>[2x]MSEFNITETYLRFLEEDTEMTMPIAAIEALVTLLRIKTPETAAEMINTIKSSTEELIKSIPNSVSLRAGCDIFMRFVLRNLHLYGDWENCKQHLIENGQLFVSRAKKSRNKIAEIGVDFIADDDIILVHGYSRAVFSLLNHAANKFIRFRCVVTESRPSKQGNQLYTLLEQKGIPVTLIVDSAVGAVIDKVDKVFVGAEGVAESGGIINLVGTYSVGVLAHNARKPFYVVTESHKFVRMFPLSSDDLPMAGPPLDFTRRTDDLEDALRGPTIDYTAQEYITALITDLGVLTPSAVSEELIKMWYD;>[2x]MSSQAFTSVHPNAATSDVNVTIDTFVAKLKRRQVQGSYAIALETLQLLMRFISAARWNHVNDLIEQIRDLGNSLEKAHPTAFSCGNVIRRILAVLRDEVEEDTMSTTVTSTSVAEPLISSMFNLLQKPEQPHQNRKNSSGSSSMKTKTDYRQVAIQGIKDLIDEIKNIDEGIQQIAIDLIHDHEILLTPTPDSKTVLKFLITARERSNRTFTVLVTEGFPNNTKNAHEFAKKLAQHNIETLVVPDSAVFALMSRVGKVIIGTKAVFVNGGTISSNSGVSSVCECAREFRTPVFAVAGLYKLSPLYPFDVEKFVEFGGSQRILPRMDPRKRLDTVNQITDYVPPENIDIYITNVGGFNPSFIYRIAWDNYKQIDVHLDKNKA;>[2x]MSIQAFVFCGKGSNLAPFTQPDFPFQTQNKDSTAATSGDKLNELVNSALDSTVINEFMQHSTRLPKALLPIGNRPMIEYVLDWCDQADFKEISVVAPVDEIELIESGLTSFLSLRKQQFELIYKALSNSNHSHHLQDPKKINFIPSKANSTGESLQKELLPRINGDFVILPCDFVTDIPPQVLVDQFRNRDDNNLAMTIYYKNSLDSSIDKKQQQKQKQQQFFTVYSENEDSERQPILLDVYSQRDVTKTKYLQIRSHLLWNYPNLTVSTKLLNSFIYFCSFELCQLLKLGPQSMSRQASFKDPFTGNQQQQNPPTTDDDEDRNHDDDDDYKPSATSIQPTYFKKKNDLILDPINCNKSLSKVFRDLSRRSWQHSKPREPIGIFILPNETLFIRANNLNAYMDANRFVLKIKSQTMFTKNIQIQSAAIGADAIVDPKCQISAHSNVKMSVLGTQANIGSRCRVAGSLLFPGVHLGDEVILENCIIGPMAKIGSKCKLSNCYIEGHYVVEPKNNFKGETLANVYLDEDEEDELIYDDSVIAGESEIAEETDSDDRSDEDSDDSEYTDEYEYEDDGLFER;>MSESEAKSRSATPPSKAKQATPTTTAAANGEKKLTNKELKELKKQEKAAKRAAMKQANGISIEQQQQQAQMKKEKKQLQREQQQKREQKQKNANKKKQNERNVKKSTLFGHLETTEERRATILALTSAVSSPKTSRITAAGLMVPVVASALSGSNVLTASSLMPVGPNASSTVSASAPASTTTTLPASSAALSAGTSSASTNTPTAIQQEIASSNASDVAKTLASISLEAGEFNVIPGISSVIPTVLEQSFDNSSLISSVKELLLNKDLIHPSILLLTSHLAHYKIVGSIPRCIAMLEVFQIVIKDYQTPKGTTLSRNLTSYLSHQIDLLKKARPLSVTMGNAIRWLKQEISLIDPSTPDKAAKKDLCEKIGQFAKEKIELADQLIIDNASTQIEESTTIVTYGSSKVLTELLLHNAISLKKNIKVIVVDSRPLFEGRKMAETLRNAGVNVMYALITSLDTIFNMDVDYVFLGAHSILSNGFLYSRAGTAMLAMSAKRRNIPVLVCCESLKFSQRVQLDSVTFNELADPNDLVNIDYENPVERRGNKGALLNQFIKERKFEKKKLAMENKPKGNKIGGKKGSEGESKDASNEEDSNSKNILDGWQELPSLNIVNILYDLTPPEYIKKVITEFGALPPSSVPVILREYKGSA[2x];>[2x]MAGKKGQKKSGLGNHGKNSDMDVEDRLQAVVLTDSYETRFMPLTAVKPRCLLPLANVPLIEYTLEFLAKAGVHEVFLICSSHANQINDYIENSKWNLPWSPFKITTIMSPEARCTGDVMRDLDNRGIITGDFILVSGDVLTNIDFSKMLEFHKKMHLQDKDHISTMCLSKASTYPKTRTIEPAAFVLDKSTSRCIYYQDLPLPSSREKTSIQIDPELLDNVDEFVIRNDLIDCRIDICTSHVPLIFQENFDYQSLRTDFVKGVISSDILGKHIYAYLTDEYAVRVESWQTYDTISQDFLGRWCYPLVLDSNIQDDQTYSYESRHIYKEKDVVLAQSCKIGKCTAIGSGTKIGEGTKIENSVIGRNCQIGENIRIKNSFIWDDCIIGNNSIIDHSLIASNATLGSNVRLNDGCIIGFNVKIDDNMDLDRNTKISASPLKNAGSRMYDNESNEQFDQDLDDQTLAVSIVGDKGVGYIYESEVSDDEDSSTEACKEINTLSNQLDELYLSDDSISSATKKTKKRRTMSVNSIYTDREEIDSEFEDEDFEKEGIATVERAMENNHDLDTALLELNTLRMSMNVTYHEVRIATITALLRRVYHFIATQTLGPKDAVVKVFNQWGLLFKRQAFDEEEYIDLMNIIMEKIVEQSFDKPDLILFSALVSLYDNDIIEEDVIYKWWDNVSTDPRYDEVKKLTVKWVEWLQNADEESSSEEE;>MSTSHCRFYENKYPEIDDIVMVNVQQIAEMGAYVKLLEYDNIEGMILLSELSRRRIRSIQKLIRVGKNDVAVVLRVDKEKGYIDLSKRRVSSEDIIKCEEKYQKSKTVHSILRYCAEKFQIPLEELYKTIAWPLSRKFGHAYEAFKLSIIDETVWEGIEPPSKDVLDELKNYISKRLTPQAVKIRADVEVSCFSYEGIDAIKDALKSAEDMSTEQMQVKVKLVAAPLYVLTTQALDKQKGIEQLESAIEKITEVITKYGGVCNITMPPKAVTATEDAELQALLESKELDNRSDSEDDEDESDDE[2x];>[2x]MSDLQDQEPSIIINGNLEPVGEPDIVEETEVVAQETQETQDADKPKKKVAFTGLEEDGETEEEKRKREFEEGGGLPEQPLNPDFSKLNPLSAEIINRQATINIGTIGHVAHGKSTVVRAISGVQTVRFKDELERNITIKLGYANAKIYKCQEPTCPEPDCYRSFKSDKEISPKCQRPGCPGRYKLVRHVSFVDCPGHDILMSTMLSGAAVMDAALLLIAGNESCPQPQTSEHLAAIEIMKLKHVIILQNKVDLMREESALEHQKSILKFIRGTIADGAPIVPISAQLKYNIDAVNEFIVKTIPVPPRDFMISPRLIVIRSFDVNKPGAEIEDLKGGVAGGSILNGVFKLGDEIEIRPGIVTKDDKGKIQCKPIFSNIVSLFAEQNDLKFAVPGGLIGVGTKVDPTLCRADRLVGQVVGAKGHLPNIYTDIEINYFLLRRLLGVKTDGQKQAKVRKLEPNEVLMVNIGSTATGARVVAVKADMARLQLTSPACTEINEKIALSRRIEKHWRLIGWATIKKGTTLEPIA;>MSSDLAAELGFDPALKKKKKTKKVIPDDFDAAVNGKENGSGDDLFAGLKKKKKKSKSVSADAEAEKEPTDDIAEALGELSLKKKKKKTKDSSVDAFEKELAKAGLDNVDAESKEGTPSANSSIQQEVGLPYSELLSRFFNILRTNNPELAGDRSGPKFRIPPPVCLRDGKKTIFSNIQDIAEKLHRSPEHLIQYLFAELGTSGSVDGQKRLVIKGKFQSKQMENVLRRYILEYVTCKTCKSINTELKREQSNRLFFMVCKSCGSTRSVSSIKTGFQATVGKRRRM[2x]

For multiple rounds of initiation to occur, the GDP on eIF2 has to be exchanged for GTP. This reaction is catalysed by a guanine nucleotide exchange factor (GEF) eIF2B. Here we have determined a cryoEM structure of eIF2B in complex with the GDP-bound form of eIF2 phosphorylated at Ser51 on the α subunit, which sheds light on the molecular interactions between the two molecules and provides a basis for understanding the regulation of translation by eIF2α phosphorylation. The structure consists of two eIF2 molecules bound to opposite sides of the eIF2B hetero-decamer.

The structure of eIF2B–eIF2(αP) complex was determined to an overall resolution of 4.2 Å at best using the counting mode dataset only (map 1). This structure was obtained by applying a twofold C2 symmetry during EM data processing, resulting in maximum resolution for the most homogeneous parts of the model but an averaged position for the eIF2 molecules, which showed a high degree of conformational heterogeneity at the periphery of the complex. As judged by the relatively high local resolution, which reflects low local flexibility and mobility, the strongest contact consists of eIF2α domain D1 inserted between the N-terminal helix bundle domains of α and δ regulatory subunits of eIF2B. The domain is inserted between the N-terminal helix bundle domains of δ and α subunits of one set of eIF2B subunits rather than binding the central cleft of eIF2B as proposed in a previous model. The most extensive interaction surface area (844 Å2) is between the eIF2α-D1 and eIF2Bα subunits, which would explain why eIF2B mutants lacking an α subunit are not sensitive to eIF2α phosphorylation, as the major part of the binding surface with eIF2α-D1 would be lost. The density in eIF2α-D1 leading to and including the phosphorylated Ser51 is visible, however, the arginine-rich loop following this serine seems to be only partially ordered. At this resolution, we cannot establish with complete confidence the interaction partners of Ser51-P because the densities for the side chains around the residue are not absolutely clear. However, the closest residues to the phosphate on Ser51 appear to be eIF2Bα H82 and Y304 and R75 slightly further away. Furthermore, in this position the phosphate may affect the conformation of the short α-helix 58–63 after the Arg-rich loop that in turn makes contacts with the eIF2Bδ NTD in our structure. eIF2Bδ residues E377 and L381 are likely to be involved in this interaction as mutations E377K and L381Q were shown to overcome the effect of Ser51 phosphorylation, suggesting that described mutations would disrupt or weaken this interaction. eIF2α phosphorylation is known to increase its binding affinity to eIF2B38, and our structure suggests that this is due to a combination of direct contact of Ser51-P with residues in eIF2Bα (H82 and/or Y304 and/or a long electrostatic interaction with R75) as well as tighter induced interaction of the 58–63 α-helix with eIF2Bδ.>MRTQWPSPAKLNLFLYITGQRADGYHTLQTLFQFLDYGDTISIELRDDGDIRLLTPVEGVEHEDNLIVRAARLLMKTAADSGRL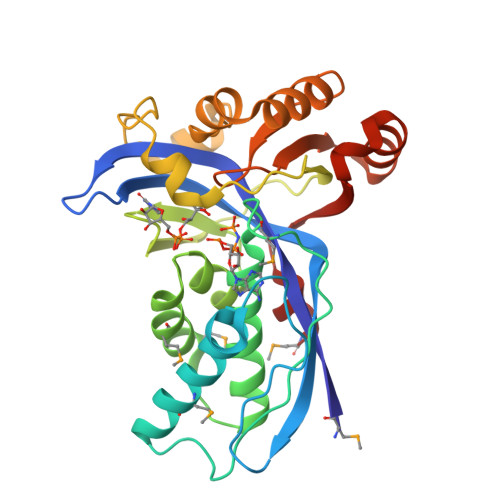PTGSGANISIDKRLPMGGGLGGGSSNAATVLVALNHLWQCGLSMDELAEMGLTLGADVPVFVRGHAAFAEGVGEILTPVDPPEKWYLVAHPGVSIPTPVIFKDPELPRNTPKRSIETLLKCEFSNDCEVIARKRFREVDAVLSWLLEYAPSRLTGTGACVFAEFDTESEARQVLEQAPEWLNGFVAKGVNLSPLHRAML[2x]>MAEQVALSRTQVCGILREELFQGDAFHQSDTHIFIIMGASGDLAKKKIYPTIWWLFRDGLLPENTFIVGYARSRLTVADIRKQSEPFFKATPEEKLKLEDFFARNSYVAGQYDDAASYQRLNSHMNALHLGSQANRLFYLALPPTVYEAVTKNIHESCMSQIGWNRIIVEKPFGRDLQSSDRLSNHISSLFREDQIYRIDHYLGKEMVQNLMVLRFANRIFGPIWNRDNIACVILTFKEPFGTEGRGGYFDEFGIIRDVMQNHLLQMLCLVAMEKPASTNSDDVRDEKVKVLKCISEVQANNVVLGQYVGNPDGEGEATKGYLDDPTVPRGST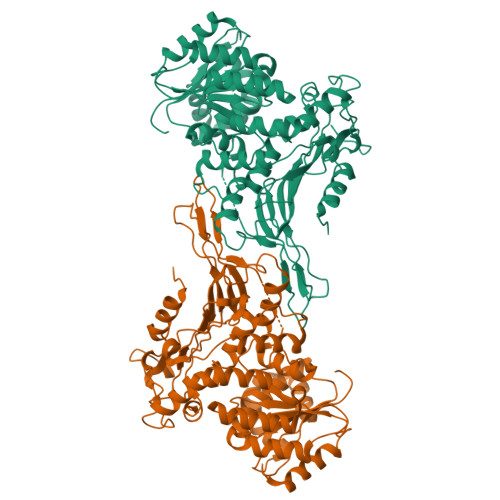TATFAAVVLYVENERWDGVPFILRCGKALNERKAEVRLQFHDVAGDIFHQQCKRNELVIRVQPNEAVYTKMMTKKPGMFFNPEESELDLTYGNRYKNVKLPDAYERLILDVFCGSQMHFVRSDELREAWRIFTPLLHQIELEKPKPIPYIYGSRGPTEADELMKRVGFQYEGTYKWVNPHKLLEHHHHHH[2x]Several natural systems exhibit ‘facilitated dissociation’, in which an effector (E) can bind to a target–host (TH) complex to form an excited ternary complex (THE)20–26 from which the target dissociates quickly. We set out to design protein systems that undergo facilitated dissociation. We use a switchable target binder (host) and a flexible effector that can rapidly bind to and switch the target–host complex to induce a large steric clash with the target, forming a strained excited ternary complex. We show here that by explicitly considering excited intermediate states when designing coupled protein systems, a broad range of facilitated dissociation systems can be designed.

We next sought to determine how the target–host–effector ternary complex deforms to resolve the designed clash. At the concentrations of the components used in the above experiments, the AS1 ternary complex is an only transiently populated excited state, but at high concentrations it becomes the dominant state (Kd,T:HE = 200 nM). In structures from two different crystals, the switch region closely matches the state Y design model, and the rest of the structure strains to resolve the structural frustration from simultaneously binding the target and occupying state Y. This strain distributes across multiple locations in the structure: the binder fusion bends, the portion of the target that directly clashes with the switch becomes disordered and the target twists at its interface, disrupting the interfacial hydrophobic packing (top) and shearing the interfacial strand pairing (bottom). Double electron–electron resonance (DEER) spectroscopy and molecular dynamics (MD) simulations suggest that the ternary complex is dynamic, with varying amounts of strain at each location. Avoiding any clash in state X while maintaining a strong clash in state Y, we sampled a variety of target + binder positions relative to the switch from AS1; rebuilt fusions between the switch and the newly located binder; and selected variants that were predicted by AlphaFold2 (AF2) to have substantial deformations spanning a variety of directions (AF2 predictions of the strained AS1 ternary complex were within 1.0 Å Cα RMSD of the target–AS1–effector crystal structure). Crystal structures throughout the facilitated dissociation process confirm our ability to design excited states and large register-shift conformational changes.

> MSGSMKEEIKRLAEELKEKTKNEEIKRLAEEAAELAERSDDPEVLEVVKKALEEALKSKNEEKIELLLLVAVLVAEAGSVDAVEEKLEIALLALKLAEESKDPRIIRGALRAAIAALRSDDPLALKTVKEALERARASKDERLIRAILAAAYAFALLAVAGASAERLKEAEAIVKELIAAAEKGASPQELVLLVIEMMVKGMGVTMETHRSGNEVKVVIKGLHESQQEVLLEAVLFAAELMGVRVRIRFKGDTVTIVV;> RKKELAKEVIETAKKLIEKLAKEE;> EEAVRRRFEELLREALAFRERTGGRRETLEHAVRLARELAEFAASHPEFNRQEAVLLAIELMVRAMGVTMETHRSGNEVKVVIKGLNIDEQVALYRAVRETSKIMGVETEIEVEGDTQTIVV A cellular pathway has been characterized that performs β-aryl ether (β-ether)3 bond cleavage using three sequential Lig enzymes. The first step in the Lig pathway is a stereospecific oxidation of the benzylic alcohol in the GGE substrate to produce β-(2-methoxyphenoxy)-γ-hydroxypropiovanillone (MPHPV), which is catalyzed by nicotinamide adenine dinucleotide (NAD+)-dependent Cα-dehydrogenases LigD, LigL, LigN, and LigO. The final step consists of a GSH-dependent lyase, LigG, that catalyzes the elimination of the GSH thioether linkage in (βR)-GS-HPV to produce glutathione disulfide (GSSG) and γ-hydroxypropiovanillone (HPV). Our structural and biochemical studies of the enzymes in the bacterial β-aryl ether cleavage pathway reveal the features important for substrate and cofactor binding and catalysis by these Lig enzymes.

The LigD and LigO enzymes catalyze the oxidation of the (αR)-substrates (αR,βR)-GGE and (αR,βS)-GGE, whereas LigL and LigN are specific for the α(S)-configured substrates (αS,βR)-GGE and (αS,βS)-GGE. We have solved the crystal structures of LigD, LigO, and LigL, which by amino acid sequence alignment belong to the short chain dehydrogenase/reductase (SDR) superfamily of enzymes. The SDR family is characterized as a large group of NAD(P)H (2′-phosphorylated NADH)-dependent enzymes displaying an α/β folding pattern containing a Rossman fold; this overall organization is seen in the LigD, LigO, and LigL crystal structures. The superposition of the LigD, LigO, and LigL structures using Cα atoms shows a root mean square deviation for LigD-LigO of 0.88 Å, for LigD-LigL of 0.70 Å, and for LigO-LigL of 0.93 Å, indicating that the enzymes display similar overall structural features. A sequence alignment of LigD, LigO, and LigL shows an identity between LigD-LigO of 40%, LigD-LigL of 38%, and LigO-LigL of 37%. In these alignments, the most sequence-divergent region is in the predicted substrate binding loop. This proposed substrate binding region is disordered in all of the crystal structures solved in the apo-form (LigD, LigO, and LigL) and in the structures of the LigD·NADH and LigO·NADH complexes.

> MKDFQDQVAFITGGASGAGFGQAKVFGQAGAKIVVADVRAEAVEKAVAELEGLGITAHGIVLDIMDREAYARAADEVEAVFGQAPTLLSNTAGVNSFGPIEKTTYDDFDWIIGVNLNGVINGMVTFVPRMIASGRPGHIVTVSSLGGFMGSALAGPYSAAKAASINLMEGYRQGLEKYGIGVSVCTPANIKSNIAEASRLRPAKYGTSGYVENEESIASLHSIHQHGLEPEKLAEAIKKGVEDNALYIIPYPEVREGLEKHFQAIIDSVAPMESDPEGARQRVEALMAWGRDRTRVFAEGDKKGA>SQFNFECFVIEDNKEVLYNSVSRFLPKKRRLTFKLS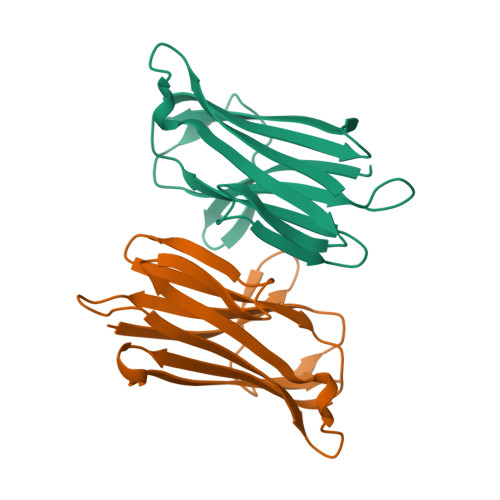IYPGPGIGDLKIIFCKRNHGQEAKDDLSEDYSISIEDNKLIRVKNADNLSLLRKDGCYVLTVPEETLFRGLHTMEVIVRGNHETLFYRNIIGVYIK[2x]>MTTNYIFVTGG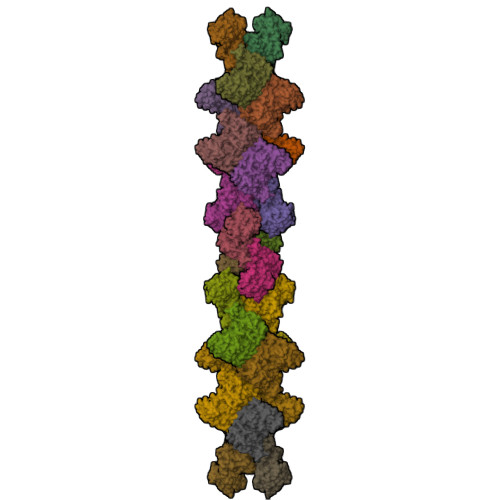VVSSLGKGIAAASLAAILEARGLNVTIMKLDPYINVDPGTMSPIQHGEVFVTEDGAETDLDLGHYERFIRTKMSRRNNFTTGRIYSDVLRKERRGDYLGATVQVIPHITNAIKERVLEGGEGHDVVLVEIGGTVGDIESLPFLEAIRQMAVEIGREHTLFMHLTLVPYMAASGEVKTKPTQHSVKELLSIGIQPDILICRSDRAVPANERAKIALFCNVPEKAVISLKDVDSIYKIPGLLKSQGLDDYICKRFSLNCPEANLSEWEQVIFEEANPVSEVTIGMVGKYIELPDAYKSVIEALKHGGLKNRVSVNIKLIDSQDVETRGVEILKGLDAILVPGGFGYRGVEGMITTARFARENNIPYLGICLGMQVALIDYARHVANMENANSTEFVPDCKYPVVALITEWRDENGNVEVRSEKSDLGGTMRLGAQQCQLVDDSLVRQLYNAPTIVERHRHRYEVNNMLLKQIEDAGLRVAGRSGDDQLVEIIEVPNHPWFVACQFHPEFTSTPRDGHPLFAGFVKAASEFQKRQAK[4x]> SMIPEVQKPLHEQLWYHGAIPRAEVAELLVHSGDFLVRESQGKQEYVLSVLWDGLPRHFIIQSLDNLYRLEGEGFPSIPLLIDHLLSTQQPLTKKSGVVLHRAVPKDKWVLNHEDLVLGEQIGRGNFGEVFSGRLRADNTLVAVKSCRETLPPDLKAKFLQEARILKQYSHPNIVRLIGVCTQKQPIYIVMELVQGGDFLTFLRT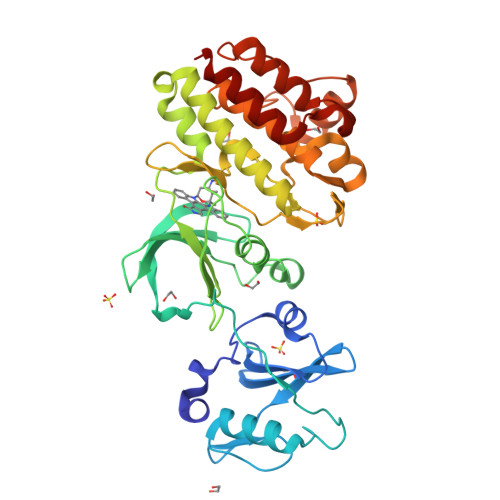EGARLRVKTLLQMVGDAAAGMEYLESKCCIHRDLAARNCLVTEKNVLKISDFGMSREEADGVYAASGGLRQVPVKWTAPEALNYGRYSSESDVWSFGILLWETFSLGASPYPNLSNQQTREFVEKGGRLPCPELCPDAVFRLMEQCWAYEPGQRPSFSTIYQELQSIRKRHR> MLAREAQNIQNPALGAALVWRFCCGYVKTNRVSAPPPLPFLFLVLPIILHQET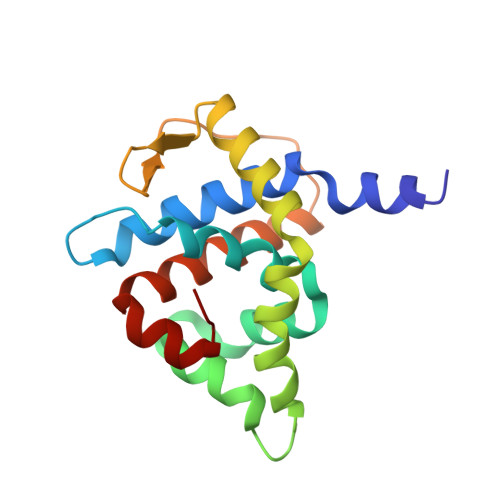SEFVKRTYKSSGLRAFAAKFGDSSVSKQDLLFQIHERSIRWRQLSLRSIELAVASDLLKLQDGSDVIPLSKTKARGLSDEVKTLMDLAEKLGSWFGELSIHEVVTTLKVKL2'-azido-2',5'-dideoxy-5'-[({5-[(3aS,4S,6aR)-2-oxohexahydro-1H-thieno[3,4-d]imidazol-4-yl]pentanoyl}sulfamoyl)amino]adenosine | C20 H28 N12 O6 S2 | 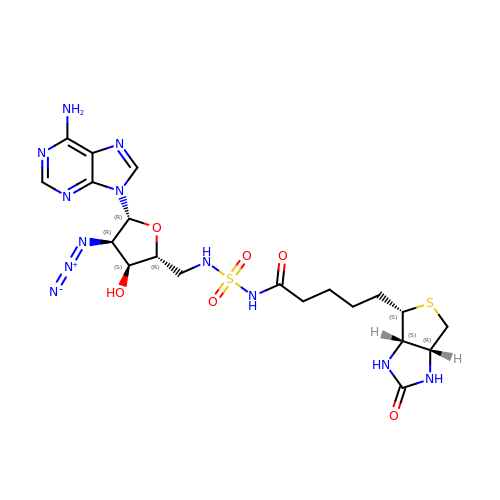ADVDUOWDPHQFNE-FALSPVJTSA-N>[2x]IVRPPFTYATLIRQAIMESSDRQLTLNEIYSWFTRTFAYFRRNAATWKNAVRHNLSLHKCFVRVENVKGAVWTVDEVEYQKRRSQKITGSPTL;>[2x]ASLPPLEWPLSSQSGSYELRIEVQPKPHHRAHYETEGSRGAVKAPTGGHPVVQLHGYMENKPLGLQIFIGTADERILKPHAFYQVHRI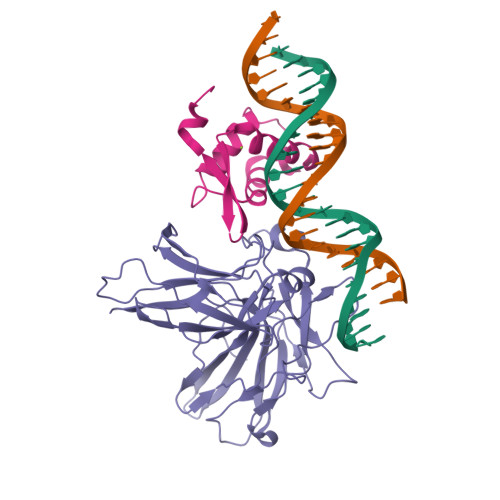TGKTVTTTSYEKIVGNTKVLEIPLEPKNNMRATIDCAGILKLRNADIELRKGETDIGRKNTRVRLVFRVHIPESSGRIVSLQTASNPIECSQRSAHELPMVERQDTDSCLVYGGQQMILTGQNFTSESKVVFTEKTTDGQQIWEMEATVDKDKSQPNMLFVEIPEYRNKHIRTPVKVNFYVINGKRKRSQPQHFTYHPV>SHMDLTYAYLVGLFEGDGYFSITKKGKYLTYELGIELSIKDVQLIYKIKDILGVGKVSFRKRNEIEMVSLRIRDKNHLKNFILPIFDKYPMLSNKQYDYLRFKDALLSNIIYSDDLPEYARSNESINSVDSIINTSYFSAWLVGFIEAEGCFSTYKLNKDDDYLIASFDIAQKDGDILISAIHKYLSFTTKIYLDKTNCSR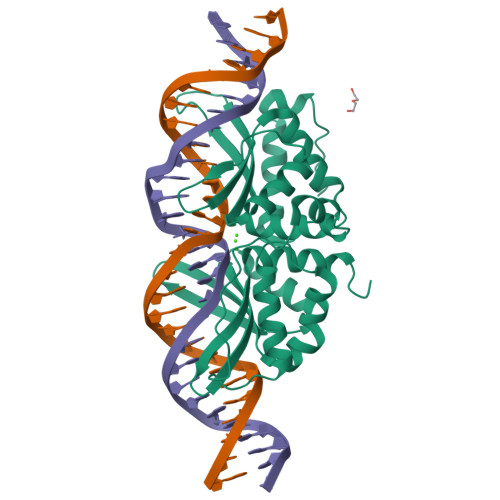LKVTGVRSVKNVVKFIQGAPVKLLGNKKLQYKLWIKQLRKISRYSEKIQLPSNY[2x]>[2x]MVEEFKVTPWEVEGVVDYDKLIKHFGTSPLTEDLLEKTAELTKSELPIFFRRKFFFSHRDYDLILKDYEEGRGFFLY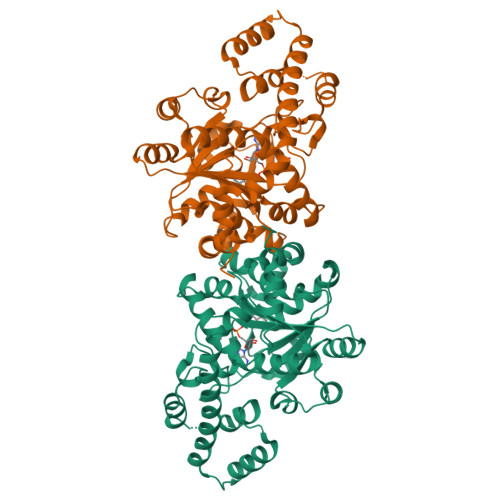TGRGPSGPMHIGHIIPFFATKWLQEKFGVNLYIQITDDEKFLFKENLTFDDTKRWAYDNILDIIAVGFDPDKTFIFQNSEFTKIYEMAIPIAKKINFSMAKAVFGFTEQSKIGMIFFPAIQIAPTFFERKRCLIPAAIDQDPYWRLQRDFAESLGYYKTAALHSKFVPSLTSLSGKMSASKPETAIYLTDSPEDVEKKVWKFTLTGGRPTLKEQREKGGEPEKCVVFKWLEIFFEEDDKKLKERYYACKNGELTCGECKRYLISKIQEFLKEHQRRRKKAEKLVEKFKYTGKLAQEMWNEAIPEPLKRSHHHHHH>[3x]QIAAHVISEASSKTTSVLQWAEKGYYTM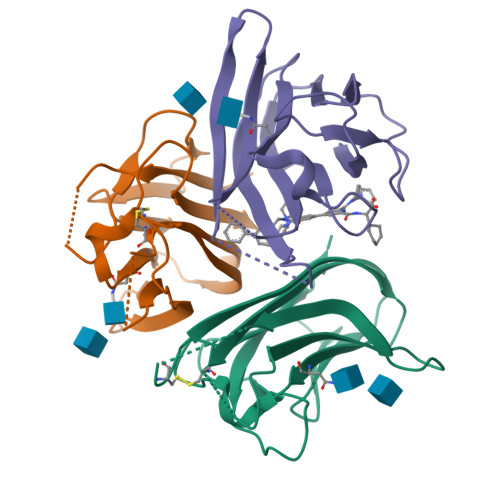SNNLVTLENGKQLTVKRQGLYYIYAQVTFCSNREASSQAPFIASLCLKSPGRFERILLRAANTHSSAKPCGQQSIHLGGVFELQPGASVFVNVTDPSQVSHGTGFTSFGLLKL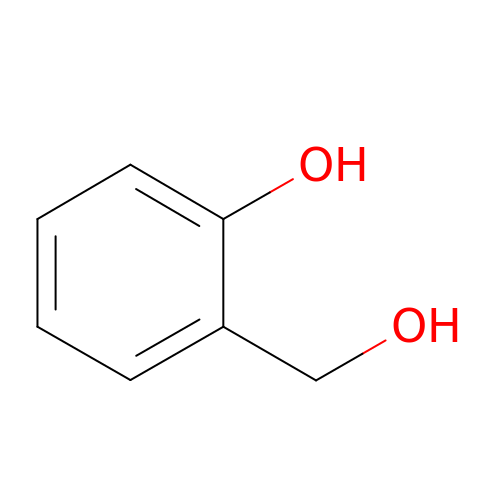2-(hydroxymethyl)phenol | C7 H8 O2 | CQRYARSYNCAZFO-UHFFFAOYSA-N>GSAEALNNLGNVYRKQGDYQKAIEYYQKALELDPNNAEALNNLGNVYRKQGDYQKAIEYYQKALELDPNNAEALNNLGNVYRKQGDYQKAIEYYQKALELDPNNAEALNNLGNVYRKQGDYQKAIEYYQKA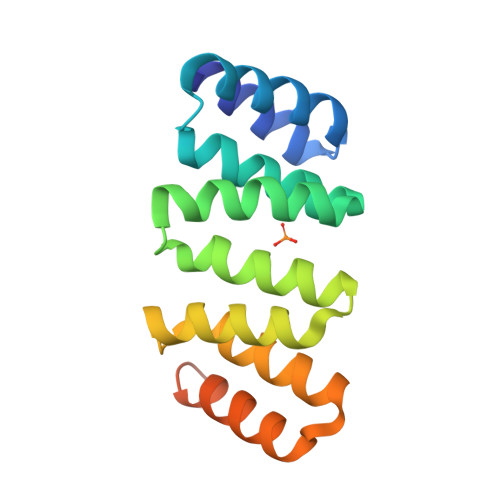LELDPNNAEALNNLGNVQRKQG[2x]> MMDLVLEEDVTVPGTLSGCSGLVPSVPDDLDGINPNAGLGNGLLPNVSEETVSPTRARNMKDFENQITELKKENFNLKLRIYFLEERMQQEFHGPTEHIYKTNIELKVEVESLKRELQEREQLLIKASKAVESLAEAGGSEIQRVKEDARKKVQQVEDLLTKRILLLEKDVTAAQAELEKAFAGTETEKALRLRLESKLSEMKKMHEGDLAMALVLDEKDRLIEELKLSLKSKEALIQCLKEEKSQMACPDENVSSGELRGLCAAPREEKERETEAAQMEHQKERNSFEERIQALEEDLREKEREIATEKKNSLKRDKAIQGLTMALKSKEKKVEELNSEIEKLSAAFAKAREALQKAQTQEFQGSEDYETALSGKEALSAALRSQNLTKSTENHRLRRSIKKITQELSDLQQERERLEKDLEEAHREKSKGDCTIRDLRNEVEKLRNEVNEREKAMENRYKSLLSESNKKLHNQEQVIKHLTESTNQKDVLLQKFNEKDLEVIQQNCYLMAAEDLELRSEGLITEKCSSQQPPGSKTIFSKEKKQSSDYEELIQVLKKEQDIYTHLVKSLQESDSINNLQAELNKIFALRKQLEQDVLSYQNLRKTLEEQISEIRRREESFSLYSDQTSYLSICLEENNRFQVEHFSQEELKKKVSDLIQLVKELYTDNQHLKKTIFDLSCMGFQGNGFPDRLASTEQTEEAKKSRLPILIKPSRSLGNMYRLPATQEVVTQLQSQILELQGELKEFKTCNKQLHQKLILAEAVMEGRPTPDKTLLNAQPPVGAAYQDSPGEQKGIKTTSSVWRDKEMDSDQQRSYEIDSEICPPDDLASLPSCKENPEDVLSPTSVATYLSSKSQPSAKVSVMGTDQSESINTSNETEYLKQKIHDLETELEGYQNFIFQLQKHSQCSEAIITVLCGTEGAQDGLSKPKNGSDGEEMTFSSLHQVRYVKHVKILGPLAPEMIDSRVLENLKQQLEEQEYKLQKEQNLNMQLFSEIHNLQNKFRDLSPPR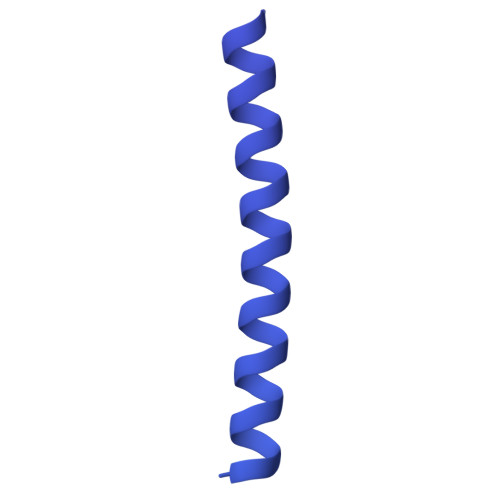YDSLVQSQARELSLQRQQIKDGHGICVISRQHMNTMIKAFEELLQASDVDYCVAEGFQEQLNQCAELLEKLEKLFLNGKSVGVEMNTQNELMERIEEDNLTYQHLLPESPEPSASHALSDYETSEKSFFSRDQKQDNETEKTSVMVNSFSQDLLMEHIQEIRTLRKRLEESIKTNEKLRKQLERQGSEFVQGSTSIFASGSELHSSLTSEIHFLRKQNQALNAMLIKGSRDKQKENDKLRESLSRKTVSLEHLQREYASVKEENERLQKEGSEKERHNQQLIQEVRCSGQELSRVQEEVKLRQQLLSQNDKLLQSLRVELKAYEKLDEEHRRLREASGEGWKGQDPFRDLHSLLMEIQALRLQLERSIETSSTLQSRLKEQLARGAEKAQEGALTLAVQAVSIPEVPLQPDKHDGDKYPMESDNSFDLFDSSQAVTPKSVSETPPLSGNDTDSLSCDSGSSATSTPCVSRLVTGHHLWASKNGRHVLGLIEDYEALLKQISQGQRLLAEMDIQTQEAPSSTSQELGTKGPHPAPLSKFVSSVSTAKLTLEEAYRRLKLLWRVSLPEDGQCPLHCEQIGEMKAEVTKLHKKLFEQEKKLQNTMKLLQLSKRQEKVIFDQLVVTHKILRKARGNLELRPGGAHPGTCSPSRPGS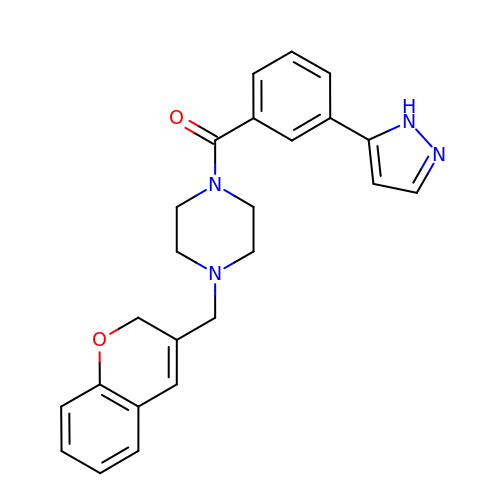[4-(2H-chromen-3-ylmethyl)piperazin-1-yl]-[3-(1H-pyrazol-5-yl)phenyl]methanone | C24 H24 N4 O2 | WZSVVCINTGQIRF-UHFFFAOYSA-N> LEERATGGYVQNPSGSASFTMYSGCGSPACGETASGYTAAMNQLSFGAGPGAGAGDACGRCFALTGTADPYS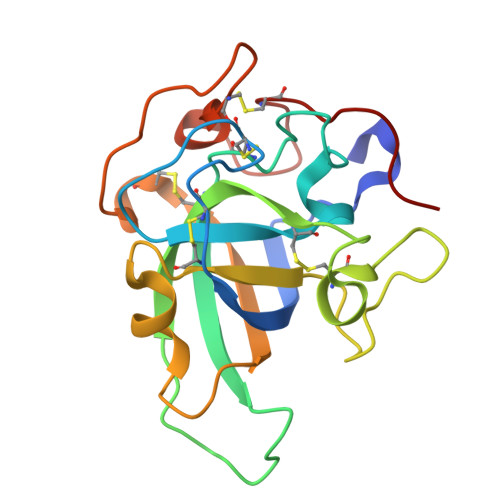PSYTGPFHTIVVKVTDLCPVAGNQEWCGQTTSNPNNQHGEPVHFDICEDTGGAGAFFPSGHGALTGTYREVSCSQWSGSDGSPLWTGACLSGESAANWPSTACGNKGTAPS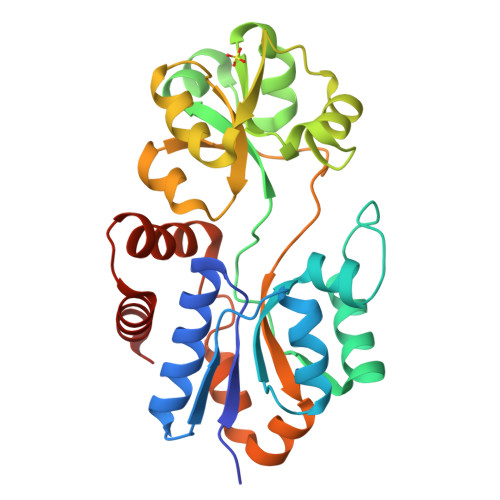>[2x]RNAIEEKPLVVATKPSSEQYILGEILSLLLEKHHIPIKRAFGIGGGTMNIHPALIRGDFDLYVEYTGTAWVNTLKNPLTQKVDFETIKKRYEKEFNLLWVGLLGFNNTYSLAISKEDAQKYAIETFSDLAFHSPNFDFGAEFDFFEREDAFKGLMKAYRFHFRSLHEMDINLRYKSFESHKINALDVFTTDAQIKELDLKVLKDDKGFFPNYQAGIVIRKETIKKYPEALKILEKLDSKINDETMQDLNYQVEVLKKSPKIVAKDFLERLGL1-~{tert}-butyl-3-[1-[(2~{S})-3-(3-carbamimidoylphenyl)-2-[[3-[3-fluoranyl-4-(hydroxymethyl)phenyl]phenyl]sulfonylamino]propanoyl]piperidin-4-yl]urea 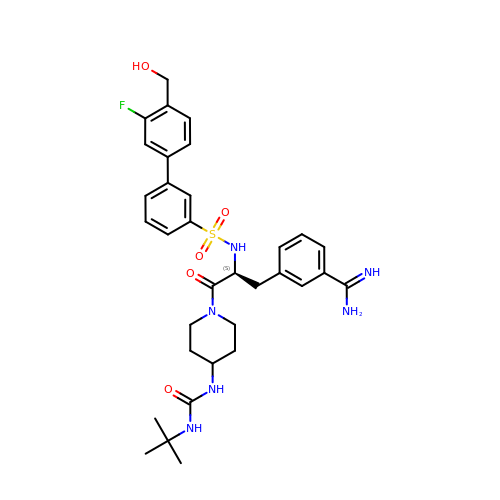| C33 H41 F N6 O5 S | FQLCVDCDDCIBQS-LJAQVGFWSA-N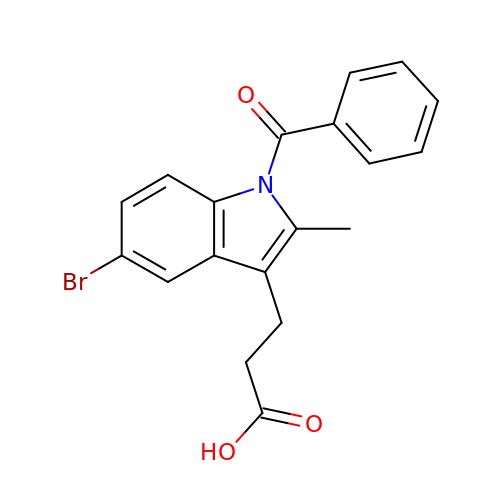3-[5-bromanyl-2-methyl-1-(phenylcarbonyl)indol-3-yl]propanoic acid | C19 H16 Br N O3 | JNJZEKLLVASXOS-UHFFFAOYSA-N>GPEIKDYWYTENEITHLLTAQLDEKKFSVQPAITFRNTALTEEMLKDYTAKGEEKNKILAEVQETIKIANLIPDKEERALMLGDAKKREEILKLSDAEREKLKNDLLRGGEAQQQINEDILNRATKDIKDNGKEAAVIPIEMGYGHWTVLVAKYDKKDNQIILTFNDSLGNSINYDGQKLPKLIDKTLGNLPNKPIIIDEQTKQQTDQSACGVFTVDNGIKIAKGQAILSTEESKGEKGLRLREHHAQILTDAMFKQDAQWIRQQMKTNNNAPD[2x]

CE clan proteases, specific hydrolases for ubiquitin-like modifications (SUMO and NEDD8) in eukaryotes, reportedly serve as bacterial effector proteins with deSUMOylase, deubiquitinase, or, even, acetyltransferase activities. Here, we characterize bacterial CE protease activities, revealing K63-linkage-specific deubiquitinases in human pathogens, such as Salmonella, Escherichia, and Shigella, as well as ubiquitin/ubiquitin-like cross-reactive enzymes in Chlamydia, Rickettsia, and Xanthomonas. Five crystal structures, including ubiquitin/ubiquitin-like complexes, explain substrate specificities and redefine relationships across the CE clan. A comparison to the previously determined SENP2-SUMO2 and NEDP1∼NEDD8 complexes (Reverter and Lima, 2004, Reverter et al., 2005, Shen et al., 2005) revealed differences among bacterial CE DUBs in three variable regions (VRs) near the substrate binding (S1) site that were arranged around a structurally conserved helix (constant region, CR).

We determined high-resolution crystal structures of the CE clan effectors SseL, RickCE, and ChlaDUB1. To this, we added entirely uncharacterized CE clan proteins RickCE (Rickettsia bellii, GenBank: ABE04279.1), LegCE (Legionella pneumophila ssp. pneumophila, GenBank: AAU28953.1), and ShiCE (Shigella flexneri; GenBank: EGK20985.1). Interestingly, the remaining bacterial effectors SseL, ElaD, and ShiCE are Ub-specific proteases, and ChlaDUB1 and RickCE cleave both Ub- and, to a lesser extent, NEDD8-modified peptides. In bacterial examples, the analogous region is either disordered in the absence of substrate (SseL) or not part of the crystallized construct (RickCE). In fact, RickCE has an ∼75-residue insertion at this site that forms a helical arm in the crystal structure. Matching their specificity profiles, ChlaDUB1 and RickCE can both form covalent adducts with Ub and NEDD8 suicide probes. Deletion of the inserted VR-3 helix of ChlaDUB1 or the predicted VR-1 outside the crystallized boundaries of RickCE resulted in a total loss in recognition of the Ub/Ubl probes. The Ub/NEDD8 cross-reactive enzymes ChlaDUB1 and RickCE fall into their own clade.>ARKCSLTGKWTNDLGSNMTIGAVNSRGEFTGTYITAVTATSNEIKESPLHGTQNT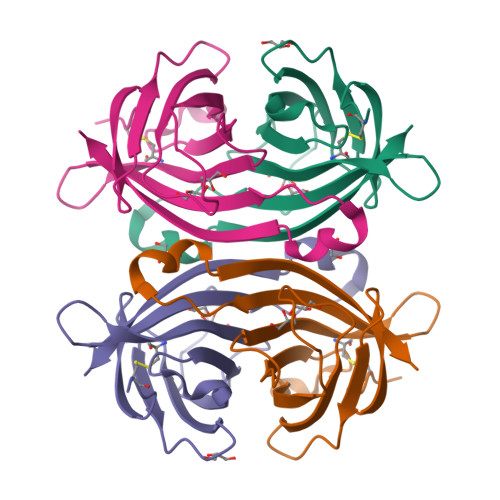INKRTQPTFGFTVNWKFSESTTVFTGQCFIDRNGKEVLKTMWLLRSSVNDIGDDWKATRVGINIFTRLRTQKE[2x]6-amino-2-[(1-naphthylmethyl)amino]-3,7-dihydro-8H-imidazo[4,5-g]quinazolin-8-one 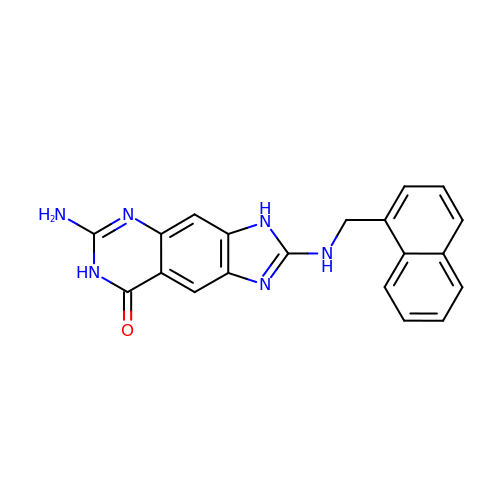| C20 H16 N6 O | MCEZMMDIEXECTI-UHFFFAOYSA-N>[4x]MADLNWISSALIKERPSADAVLAKAVLAAREQLGLTQLELAGIVGVDRSAISRWKTQGLRVDSKTGELALLLVRVYRALYALFGGQQEDMRHFLRTPNHHL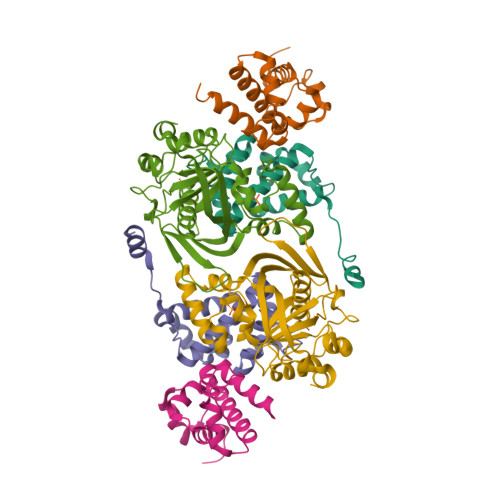AGEPLALMGQVQGLVHVLEYLDAIRGKV;>[2x]MGSSHHHHHHSQDPSEIWRQCKGERHIRPLQGRLVRLVESQDQVATLQLVDTLEEQALLEELLESSKPPVPADAEPLHYLLKTPFRYPPLRWGSRFGRRHEPSLFYAALKLETAMAESAYYRCVLWSGMVVPPPSGRILSEHASFEAGWKVERGIRLQAPPFSDHEAALTDIADYRAPQELGSAMRSAGVQAFEYRSARCPERGCNVALFTPAAFTEKRPRNLTPWLCETTAGYVAFKPAHVPGSPKIFSWELFLVDGKLPHPA(2~{S})-2-[[(2~{S})-6-[(6-fluoranylpyridin-3-yl)-methyl-amino]-1-oxidanyl-1,6-bis(oxidanylidene)hexan-2-yl]carbamoylamino]pentanedioic 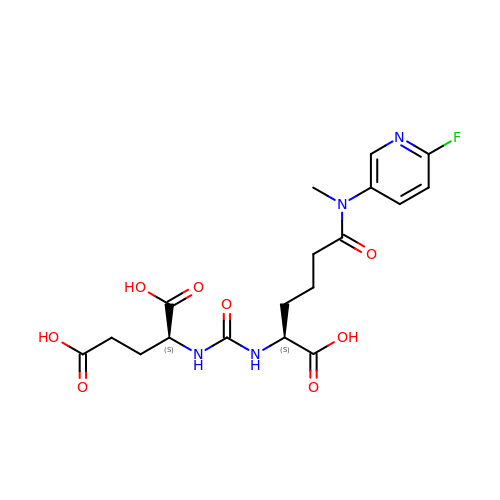acid | C18 H23 F N4 O8 | UUDMXDXHNXMSOT-RYUDHWBXSA-N>[4x]ARFEEQKLYIGGRYVEASSGATFETINPANGEVLAKVQRASREDVERAVQSAVEGQKVWAAMTAMQRSRILRRAVDILRERNDELAALETLDTGKPLAETRSVDIVTGADVLEYYAGLVPAIEGEQIPLRETSFVYTRREPLGVVAGIGAWNYPVQIALWKSAPALAAGNAMIFKPSEVTPLTALKLAEIYTEAGVPDGVFNVLTGSGREVGQWLTEHPLIEKISFTGGTSTGKKVMASASSSSLKEVTM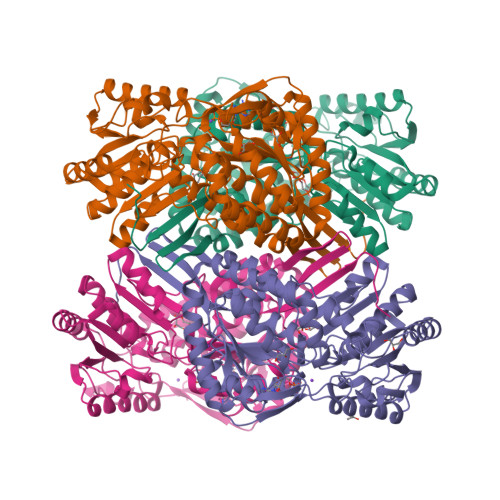ALGGKSPLIIFPDADLDRAADIAVMANFFSSGQVCTNGTRVFIHRSQQARFEAKVLERVQRIRLGDPQDENTNFGPLVSFPHMESVLGYIESGKAQKARLLCGGERVTDGAFGKGAYVAPTVFTDCRDDMTIVREEIFGPVMSILVYDDEDEAIRRANDTEYGLAAGVVTQDLARAHRAIHRLEAGICWINTWGESPAEMPVGGYKQSGVGRENGLTTLAHYTRIKSVQVELGDYASVF>GPKLREVKYELDTKVSELSHKLGSSEGSNRSLEEETARLRSLNQQLSSSKHELEIQLNEAKAKVLALDEKAQSQGDVIEQQRGRLRDMEAALRQTEQRCADLR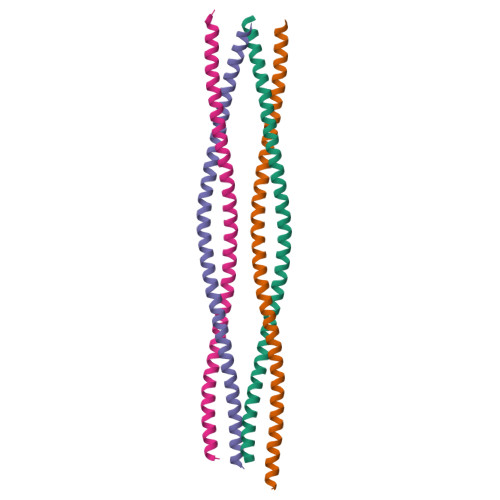DTLASAEGRAKEA[8x]>SVLLSRELHPVAPLLDNLISALNKVYQRKGVNISMDISPEISFVGEQNDFVEVMGNVLDNACKYCLEFVEISARQTDDHLHIFVEDDGPGIPHSKRSLVFDRGQRADTLRPGQGVGLAVAREIT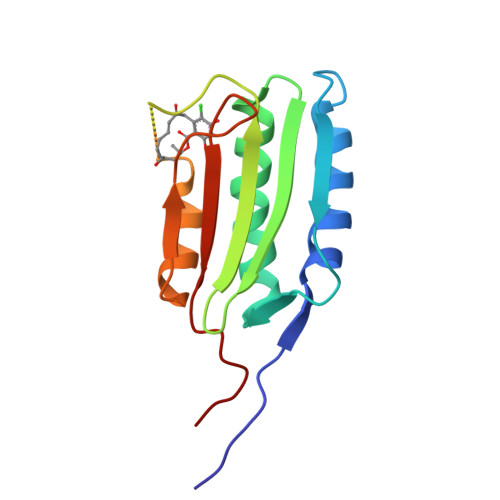EQYAGQIIASDSLLGGARMEVVFGRQHPTQKEE[3x]>[4x]MEEKALIGIEDFLKVDLRVAKVLSAERVEGSEKLLKLT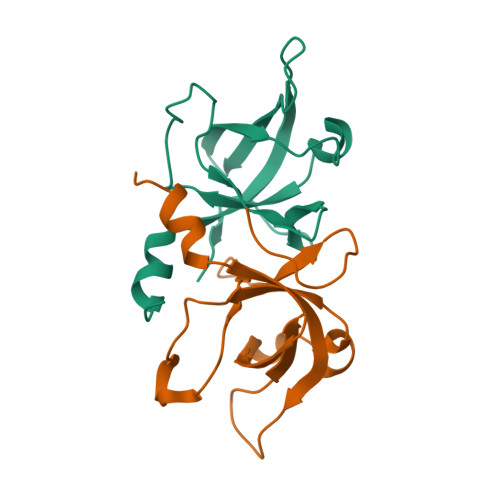LSLGDEERTVVAGIAKYYTPEELVGKKIVIVANLKPRKIFGIESQGMILAASDGENLSVIVPDRDVKEGAKLS> MAEAGLRGWLLWALLLRLAQSEPYTTIHQPGYCAFYDECGKNPELSGSLMTLSNVSCLSNTPARKITGDHLILLQKICPRLYTGPNTQACCSAKQLVSLEASLSITKALLTRCPACSDNFVNLHCHNTCSPNQSLFINVTRVAQLGAGQLPAVVAYEAFYQHSFAEQSYDSCSRVRVPAAATLAVGTMCGVYGSALCNAQRWLNFQGDTGNGLAPLDITFHLLEPGQAVGSGIQPLNEGVARCNESQGDDVATCSCQDCAASCPAIARPQALDSTFYLGQMPGSLVLIIILCSVFAVVTILLVGFRVAPARDKSKMVDPKKGTSLSDKLSFSTHTLLGQFFQGWGTWVASWPLTILVLSVIPVVALAAGLVFTELTTDPVELWSAPNSQARSEKAFHDQHFGPFFRTNQVILTAPNRSSYRYDSLLLGPKNFSGILDLDLLLELLELQERLRHLQVWSPEAQRNISLQDICYAPLNPDNTSLYDCCINSLLQYFQNNRTLLLLTANQTLMGQTSQVDWKDHFLYCANAPLTFKDGTALALSCMADYGAPVFPFLAIGGYKGKDYSEAEALIMTFSLNNYPAGDPRLAQAKLWEEAFLEEMRAFQRRMAGMFQVTFMAERSLEDEINRTTAEDLPIFATSYIV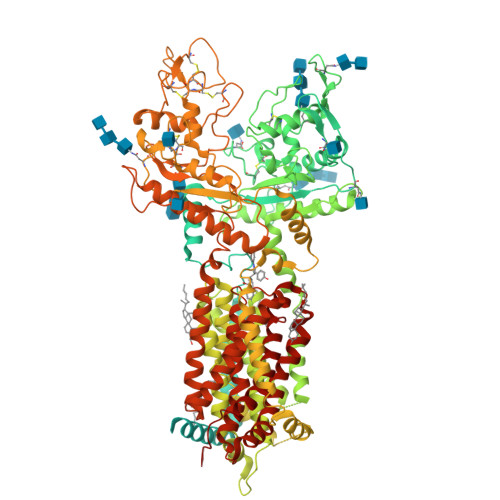IFLYISLALGSYSSWSRVMVDSKATLGLGGVAVVLGAVMAAMGFFSYLGIRSSLVILQVVPFLVLSVGADNIFIFVLEYQRLPRRPGEPREVHIGRALGRVAPSMLLCSLSEAICFFLGALTPMPAVRTFALTSGLAVILDFLLQMSAFVALLSLDSKRQEASRLDVCCCVKPQELPPPGQGEGLLLGFFQKAYAPFLLHWITRGVVLLLFLALFGVSLYSMCHISVGLDQELALPKDSYLLDYFLFLNRYFEVGAPVYFVTTLGYNFSSEAGMNAICSSAGCNNFSFTQKIQYATEFPEQSYLAIPASSWVDDFIDWLTPSSCCRLYISGPNKDKFCPSTVNSLNCLKNCMSITMGSVRPSVEQFHKYLPWFLNDRPNIKCPKGGLAAYSTSVNLTSDGQVLASRFMAYHKPLKNSQDYTEALRAARELAANITADLRKVPGTDPAFEVFPYTITNVFYEQYLTILPEGLFMLSLCLVPTFAVSCLLLGLDLRSGLLNLLSIVMILVDTVGFMALWGISYNAVSLINLVSAVGMSVEFVSHITRSFAISTKPTWLERAKEATISMGSAVFAGVAMTNLPGILVLGLAKAQLIQIFFFRLNLLITLLGLLHGLVFLPVILSYVGPDVNPAL> AELTVDQQTLLDYIMDSYSKQRMPQEITNKILKEEFSAEENFLILTEMATSHVQILVEFTKRLPGFQTLDHEDQIALLKGSAVEAMFLRSAEIFNKKLPAGHADLLEERIRKSGISDEYITPMFSFYKSVGELKMTQEEYALLTAIVILSPDRQYIKDREAVEKLQEPLLDVLQKLCKIYQPENPQHFACLLGRLTELR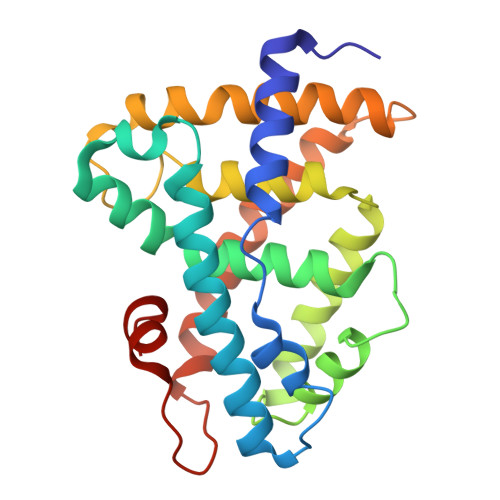TFNHHHAEMLMSWRVNDHKFTPLLCEIWDVQ>MFTKRHRITLLFNANKAYDRQVVEGVGEYLQASQSEWDIFIEEDFRARIDKIKDWLGDGVIADFDDKQIEQALADVDVPIVGVGGSYHLAESYPPVHYIATDNYALVESAFLHLKEKGVNRFAFYGLPESSGKRWATEREYAFRQLVAEEKYRGVVYQGLETAPENWQHAQNRLADWLQTLPPQTGIIAVTDARARHILQVCEHLHIPVPEKLCVIGIDNEELTRYLSRVALSSVAQGARQMGYQAAKLLHRLLDKEEMPLQRILVPPVRVIERRSTDYRSLTDPAVIQAMHYIRNHACKGIKVDQVLDAVG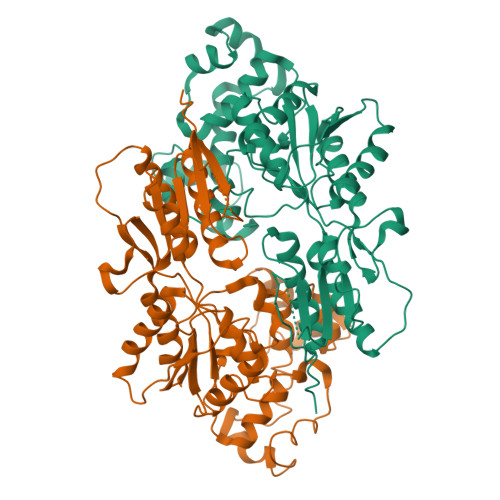ISRSNLEKRFKEEVGETIHAMIHAEKLEKARSLLISTTLSINEISQMCGYPSLQYFYSVFKKAYDTTPKEYRDVNSEVML[3x]>[2x]MTTETFVKDIKPGLKNLNLIFIVLETGRVTKTKDGHEVRTCKVADKTG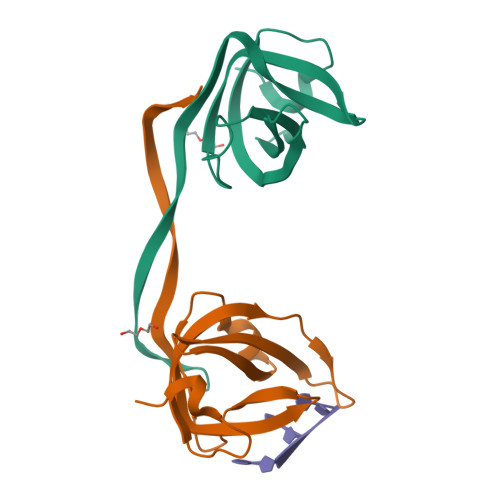SINISVWDDVGNLIQPGDIIRLTKGYASVFKGCLTLYTGRGGDLQKIGEFCMVYSEVPNFSHHHHHH>MAQNDNYIYSTEVGGVGGTPFTFMQESGTITSIKFNWSDQY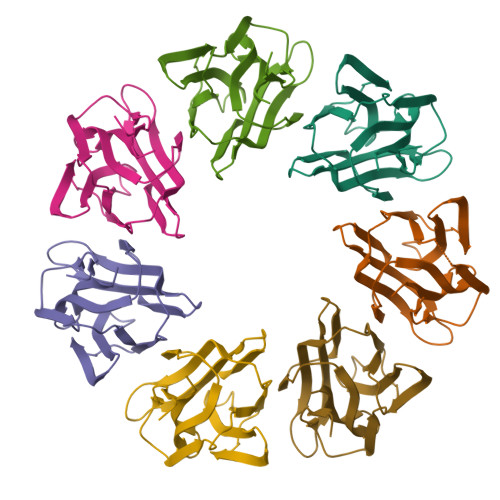KLLHHIEVKFINNANIYATGDPKGNHEVILEIDDDETIIGSVIGYKKGNDGRCTGVKLTTSKGKSIMAGYFEESLITTYTGKLAGIKGGAGSAIDRLGLIFLKK[14x]>CGTGAGGCG[4x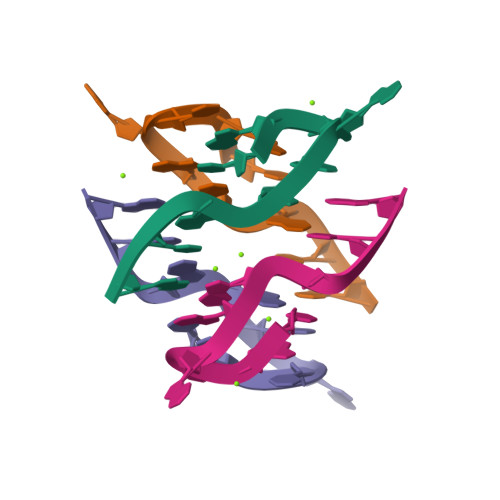]> MHHHHHHSSGLEVLFQGPGSTLVRVKKSAATLGIAIEGGANTRQPLPRIVTIQR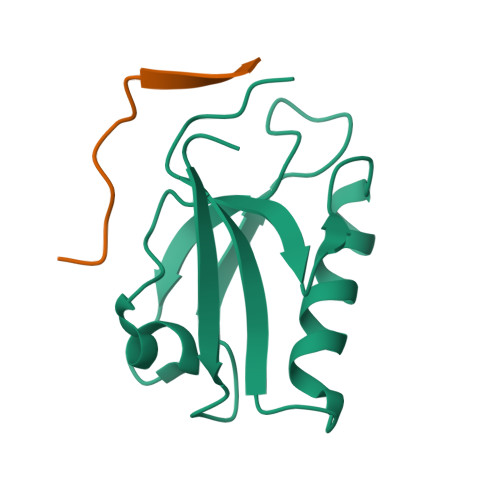GGSAHNCGQLKVGHVILEVNGLTLRGKEHREAARIIAEAFKTKDRDYIDFLVTEFNVML;> EKRLTLPPSEITLL> PTLSPEQQEMLQAFSTQSGMNLEWSQKCLQDNNWDYTRSAQ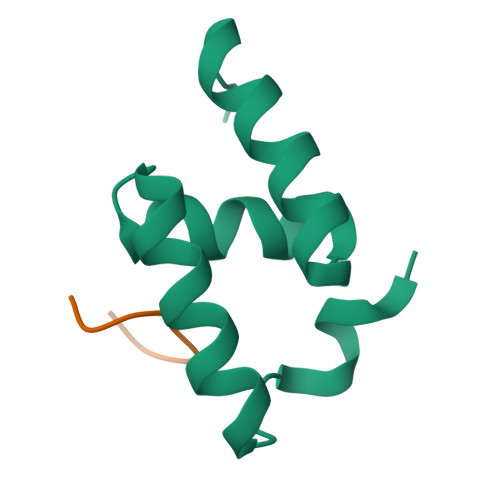AFTHLKAKGEIPEVAFMK;> DSGFSFGSK>[2x]ALAGTIIAGASLTFQVLDKVLEELGKVSRKIAVGIDNESGGTWTALNAYFRSGTTDVILPEFVPNTKALLYSGRKDTGPVATGAV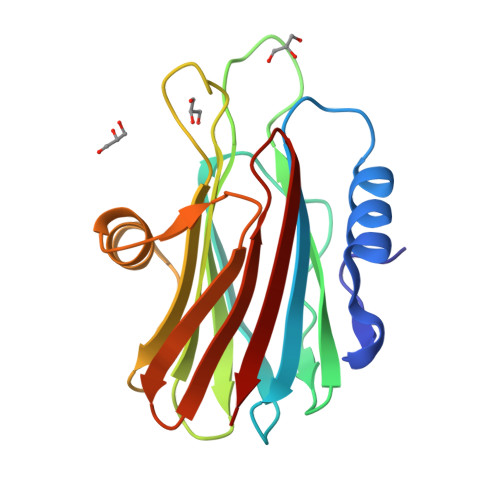AAFAYYMSSGNTLGVMFSVPFDYNWYSNWWDVKIYSGKRRADQGMYEDLYYGNPYRGDNGWHEKNLGYGLRMKGIMTSAGEAKMQIKISR> IVGGYTCGANTVPYQVSLNSGYHFCGGSLINSQWVVSAAHCYKSGIQVRLGEDNINVVEGNEQFISASKSIVHPSYNSNTLNNDIMLIKLKSAASLNSRVASISLPTSCASAGTQCLISGWGNTKSSGTSYPDVLKCLKAPILSDSSCKSAYPGQITSNMFCAGYLEGGKDSCQGDSGGPVVCSGKLQGIVSWGSGCAQKNKPGVYTKVCNYVSWIKQTIASN;> SGHH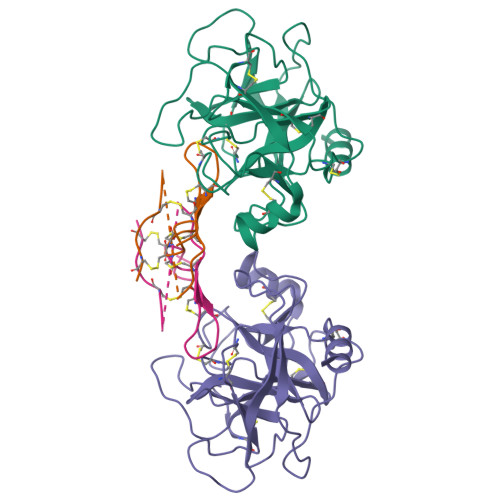DETTDEPSESSKPCCDQCSCTKSMPPKCRCSDIRLNSCHSACKSCACTYSIPAKCFCTDINDFCYEPCKSSRDDDWDN> MNKPIKNIVIVGGGTAGWMAASYLVRALQQQANITLIESAAIPRIGVGEATIPSLQKVFFDFLGIPEREWMPQVNGAFKAAIKFVNWRKSPDPSRDDHFYHLFGNVPNCDGVPLTHYWLRKREQGFQQPMEYACYPQPGALDGKLAPCLSDGTRQMSHAWHFDAHLVADFLKRWAVERGVNRVVDEVVDVRLNNRGYISNLLTKE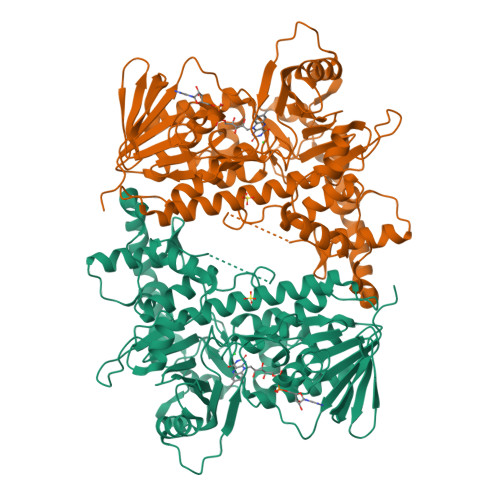GRTLEADLFIDCSGMRGLLINQALKEPFIDMSDYLLCDSAVASAVPNDDARDGVEPYTSSIAMNSGWTWKIPMLGRFGSGYVFSSHFTSRDQATADFLKLWGLSDNQPLNQIKFRVGRNKRAWVNNCVSIGLSSCFLEPLESTGIYFIYAALYQLVKHFPDTSFDPRLSDAFNAEIVHMFDDCRDFVQAHYFTTSRDDTPFWLANRHDLRLSDAIKEKVQRYKAGLPLTTTSFDDSTYYETFDYKFKNFWLNGNYYCIFAGLGMLPDRSLPLLQHRPESIEKAEAMFASIRREAERLRTSLPTNYDYLRSLRDGDAGLSRGQRGPKLAAQESL Here we report the discovery of type IV borosin natural product pathways (termed ‘split borosins’), featuring an iteratively acting α-N-methyltransferase and separate precursor peptide substrate from the metal-respiring bacterium Shewanella oneidensis. The α-N-methyltransferase SonM from Shewanella oneidensis MR-1 iteratively methylates its substrate SonA at two residues, SonA-L63 and SonA-I65, in an N-to-C terminal fashion on the core peptide. Complexes of SonM and SonA form dimers of heterodimers. A five helical bundle at the N-terminus of SonA, now referred to as the borosin binding domain (BBD; 1–53), serves as the SonA leader peptide and is homologous to a portion of the fused clasp region of OphMA.

To further test the role of the core peptide on the binding of SonA to SonM, the Ki for a BBD-only construct (SonA-BBD; 1–55) was estimated to be 3.9 μM. Indeed, one of the heterodimers is bound to the cofactor SAM, and the overall conformation is similar to the heterodimer SonM—SonA-2Me—SAH structure. The cognate SonM—SonA-BBD heterodimer is without cofactor, and shows large conformational changes as compared to the apo SonM—SonA-2Me structure. The active site binding cleft in the SonM—SonA-BBD heterodimer appears largely open, and there are diverse conformational changes compared to the other, cofactor-bound heterodimer. Most prominently, the residue SonM-Y93 that interacts with the cofactor adopts a completely different rotamer (the hydroxyl group of the side chain differs by 7.3 Å between the apo heterodimer SonM—SonA-BBD and the apo SonM—SonA-2Me structure). The top clamp that is typically observed in closed conformation in the other SonM—SonA-2Me structures, but also in OphMA and dbOphMA structures, relocates by nearly 14 Å. Indeed, a careful analysis and comparison of both conformations reveals an interaction network between the cofactor SAM, the side clamp, and the top clamp. Specifically, the binding of SAM, and in particular the ribose moiety, appears to sterically hinder and induce a conformational change for residues SonM-W166 and SonM-F99. Relocation of SonM-F99 (Domain A; ~2.8 Å) and SonM-W166 (Domain B; ~2 Å) brings both residues closer (4.8 Å in the apo structure vs. 3.4 Å) to a near-canonical π–π sandwich-stacking configuration.

>[4x]MGSLVCVGTGLQLAGQISVLSRSYIEHADIVFSLLPDGFSQRWLTKLNPNVINLQQFYAQNGEVKNRRDTYEQMVNAILDAVRAGKKTVCALYGHPGVFACVSHMAITRAKAEGFSAKMEPGISAEACLWADLGIDPGNSGHQSFEASQFMFFNHVPDPTTHLLLWQIAIAGEHTLTQFHTSSDRLQILVEQLNQWYPLDHEVVIYEAANLPIQAPRIERLPLANLPQAHLMPISTLLIPPAKKLEYNYAILAKLGIGPEDLG;>MSGLSDFFTQLGQDAQLMEDYKQNPEAVMRAHGLTDEQINAVMTGDMEKLKTLSGDSSYQSYLVISHGNGD[4x]> GDSASQAEQFLKLV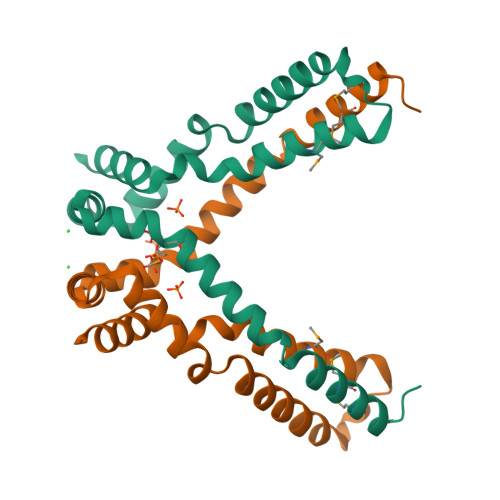HADKLTVPVYAQVQQMLAQRFAQAKAPESKKAVLERYQAKANAELDRAIGWDKIKPELIKLYTTNFTESELKDLNAFYQSPLGKKVLEKMPRLTAESAQLTQAKLQGAVEPVNKLMADMDKELGVAAPAQKKK>[3x]ANSERTFI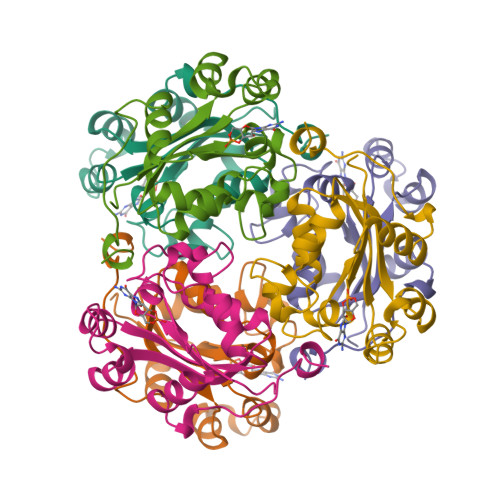AIKPDGVQRGLMGEIIKRFEQKGFRLVAMKFMRASEDLLKEHYIDLKDRPFFAGLVKYMHSGPVVAMVWEGLNVVKTGRVMLGETNPADSKPGTIRGDFCIQVGRNIIHGSDSVESAEKEIALWFRPEELVNYKSCAQNWIYE N-[5-[(3-methylphenyl)sulfamoyl]-1,3,4-thiadiazol-2-yl]naphthalene-2-carboxamide | C20 H16 N4 O3 S2 | 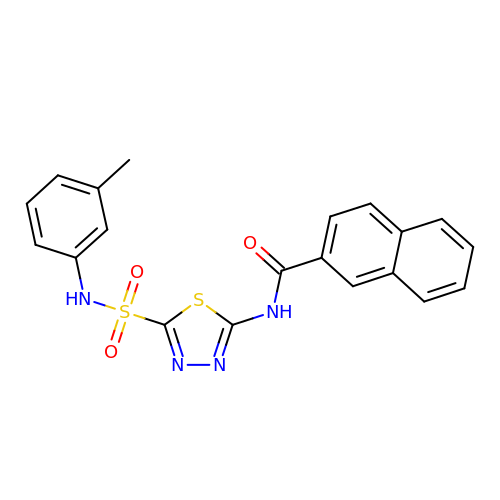SHYVRGLGJPAIBR-UHFFFAOYSA-N> MAKKTSSGRGKLPPGPTPLPVIGNILQIGIKDISKSLTNLSKVYGPVFTLYFGLKPIVVLHGYEAVKEALIDLGEEFSGRGIFPLAERANRGFGIVFSNGKKWKEIRRFSLMTLRNFGMGKRSIEDRVQEEARCLVEELRKTKASPCDPTFILGCAPCNVICSIIFHKRFDYKDQQFLNLMEKLNENIKILSSPWIQICNNFSPIIDYFPGTHNKLLKNVAFMKSYILEKVKEHQESMDMNNPQDFIDCFLMKMEKEKHNQPSEFTIESLENTAVDLFGAGTETTSTTLRYALLLLLKHPEVTAKVQEEIERVIGRNRSPCMQDRSHMPYTDAVVHEVQRYIDLLPTSLPHAVTCDIKFRNYLIPKGTTILISLTSVLHDNKEFPNPEMFDPHHFLDEGGNFKKSKYFMPFSAGKRICVGEALAGMELFLFLTSILQNFNLKSLVDPKNLDTTPVVNGFASVPPFYQLCFIPIHHHH

Mtb Decaprenylphosphoryl‐β‐d‐ribofuranose 2‐oxidase (DprE1) is a flavin adenine dinucleotide (FAD)‐dependent enzyme, which together with decaprenylphosphoryl‐d‐2‐ketoerythropentose reductase (DprE2), converts decaprenylphosphoryl‐beta‐d‐ribose (DPR) to decaprenylphosphoryl‐beta‐d‐arabinofuranose (DPA), an essential cell wall component. Multiple covalent3 and non‐covalent4 DprE1 inhibitors have been identified and showed in vitro and in vivo activities against Mtb, further validating DprE1 as an attractive anti‐tuberculosis (TB) drug target. When analyzing toxicity profiles, we noticed that many TCA1 analogs show inhibition of CYP2C9, one of six major cytochrome P450 enzymes which determine the clearance of 75 % of marketed drugs. Here we report the X‐ray crystal structures of WT DprE1, a TCA1‐resistant DprE1 mutant, and CYP2C9 in complex with TCA1 analogs.

Similar to the binding of TCA1 to DprE1, the thiophene group of TCA007 binds in a hydrophobic pocket of the 2C9 substrate binding cavity that is far from the iron of the heme cofactor where the reactive oxidant is formed, thus preventing oxygenation of the thiophene moiety. The pocket is formed by the inner surface of helix B′ and adjacent residues and hydrophobic residues on helix F across from B′ and helix G above TCA007. Mimicking the role of DprE1 Lys418, Arg108 donates H‐bonds from Nϵ to the carbonyl oxygen of the thiophene carboxamide (3.0 Å) and from Nη2 to the thiazole nitrogen (3.4 Å). Phe100, Leu102, and Phe114 form a hydrophobic pocket together with Phe476 where the carbamate group of TCA007 is bound. In contrast to DprE1, protein H‐bond donors for the carbamate are not present in this pocket, but the cavity is open to solvent and an ordered water molecule donates an H‐bond to the carbonyl of the acyl group. The pyridyl nitrogen of the pyridothiozole group is oriented toward the heme but is too distant (6.6 Å) for coordination to the heme iron. Consistent with this observation, TCA007 does not significantly alter the visible absorption spectrum of 2C9 in solution. In contrast, miconazole binds to the heme iron of 2C9 and alters the spectrum of the heme co‐factor, and competitive displacement of iron bound miconazole by TCA007 reverts the spectrum of the miconazole complex to that of the apo enzyme. This portion of the active site is also hydrophobic, but a molecule of water is evident 2.88 Å from the pyridyl nitrogen of TCA007. The water molecule is hydrogen bonded to a second water molecule that donates a lone pair of electrons to the heme iron and a H‐bond to the backbone carbonyl of Ala297. In general, the extensive hydrophobic interactions and hydrogen bonding interactions with Arg108 are likely to form the basis for the high affinity, reversible binding of TCA007 to 2C9, but these interactions also sequester TCA007 in position that reduces the likelihood of metabolism, which is consistent with absent or low rates of metabolite formation or time dependent inhibition.2-(1,5-DIDEOXYRIBOSE)-4-AMIDO-THIAZOLE 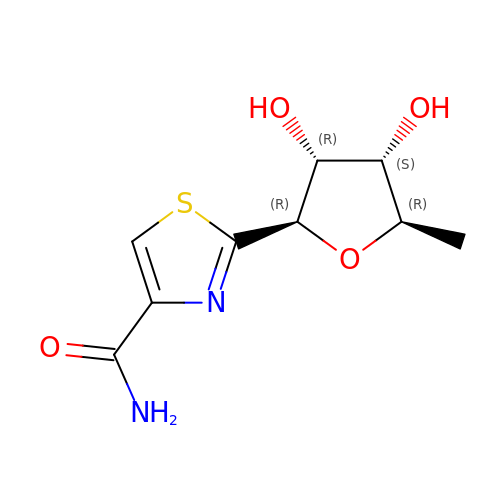| C9 H12 N2 O4 S | FQKJMVYTLPKRQR-SHUUEZRQSA-N>[3x]XGIAAIKQEHAAIKQEIAAIKQEIAA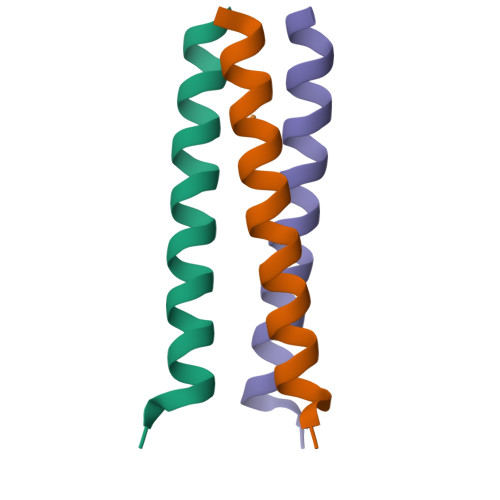IKWEGX> MGKLQKQLLEAVEHKQLRPLDVQFALTVAGDEHPAVTLAAALLSHDAGEGHVCLPLSRLENNEASHPLLATCVSEIGELQNWEECLLASQAVSRGDEPTPMILCGDRLYLNRMWCNERTVARFFNEVNHAIEVDEALLAQTLDKLFPVSDEINWQKVAAAVALTRRISVISGGPGTGKTTTVAKLLAALIQMADGERCRIRLAAPTGKAAARLTESLGKALRQLPLTDEQKKRIPEDASTLHRLLGAQPGSQRLRHHAGNPLHLDVLVVDEASMIDLPMMSRLIDALPDHARVIFLGDRDQLASVEAGAVLGDICAYANAGFTAERARQLSRLTGTHVPAGTGTEAASLRDSLCLLQKSYRFGSDSGIGQLAAAINRGDKTAVKTVFQQDFTDIEKRLLQSGEDYIAMLEEALAGYGRYLDLLQARAEPDLIIQAFNEYQLLCALREGPFGVAGLNERIEQFMQQKRKIHRHPHSRWYEGRPVMIARNDSALGLFNGDIGIALDRGQGTRVWFAMPDGNIKSVQPSRLPEHETTWAMTVHKSQGSEFDHAALILP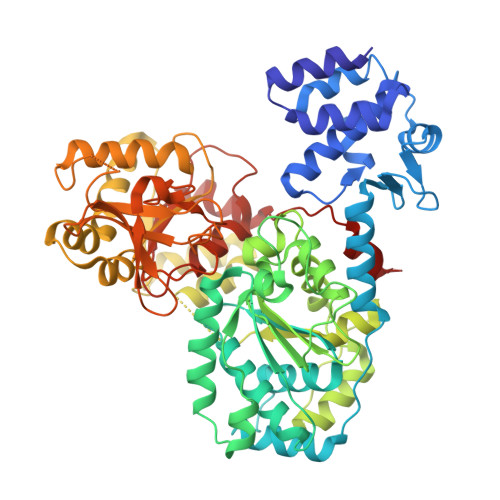SQRTPVVTRELVYTAVTRARRRLSLYADERILSAAIATRTERRSGLAALFSSRE> SENLYFQGSANAVCQ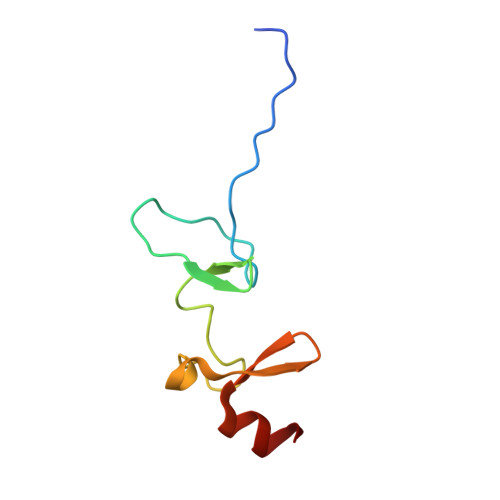RCQARFSPAERIVNSNGELYHEHCFVCAQCFRPFPEGLFYEFEGRKYCEHDFQMLFA>[2x]ESQPDPKPDELHKSSKFTGLMEYMKVLYDDNHVSAINVKSIDQFLYFDLIYSIKDTKLGNYDNVRVEFKNKDLADKYKDKYVDVFGANYYYQCYFSSSTNDINSHQTDKRKTCMYGGVT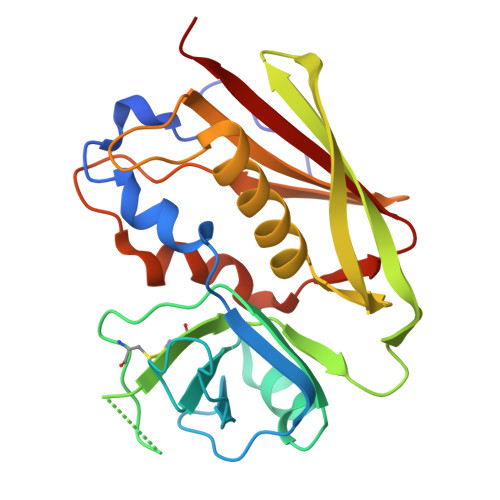EHNGNQLDKYRSITVRVFEDGKNLLSFDVQTNKKKVTAQELDYLTRHYLVKNKKLYEFNNSPYETGYIKFIENENSFWYDMMPAPGDKFDQSKYLMMYNDNKMVDSKDVKIEVYLTTKKK> SMQGNWNMGPPGGLQ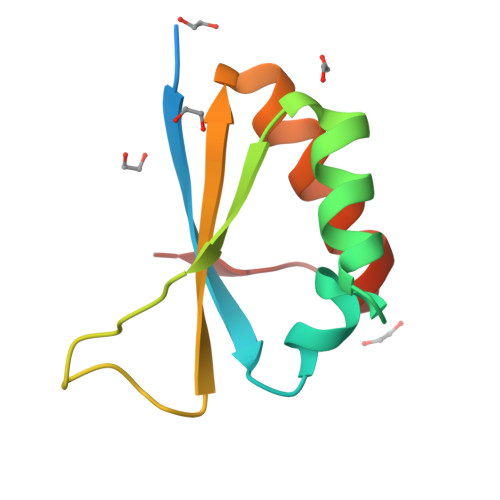EFNFIVPTGKTGLIIGKGGETIKSISQQSGARIELQRNPPPNADPNMKLFTIRGTPQQIDYARQLIEEKIGGPVNPLG N-[(3R,4S,5R,6R,7R)-3,5,6-trihydroxy-7-(hydroxymethyl)azepan-4-yl]acetamide 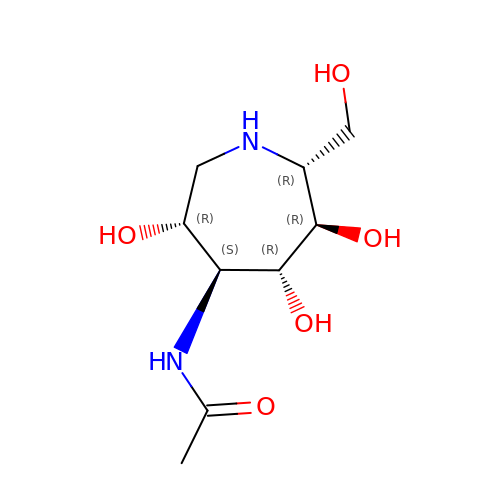| C9 H18 N2 O5 | RJAFVDFBXXHCRJ-SYHAXYEDSA-N> DSFLQRYSSDP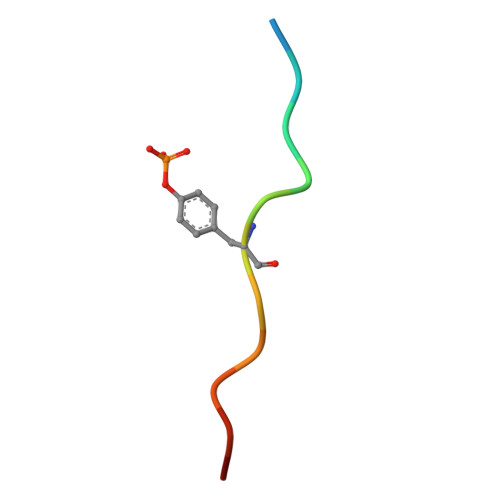TG> MGSSHHHHHHSQDPANRNVPIPRRQLYIGGEWREPVKKNRIPIINPATEEIIGDIPAATAEDVDIAVEAARKAIARDDWGSTTGAQRAKYLRAIAAKVLEKKSVLATLESLDSGKTLYESAADMDDVAGCFEYYAGLAEALDSRRMTPVNLNSDSYKSYVLREPLGVVGLITPWNYPLLMAIWKVAPALAAGCAAILKPSELASITCLELGEICREIGLPSGALNILTGLGPEAGGPLASHPHVDKISFTGSGPTGSKIMTAAAQLVKPVSLALGGKSPIVVFDDIDNLDIAAEWTLFGIFANTGQVCSATSRLIVQENIASAFMDRLLKWTKNIKISDPL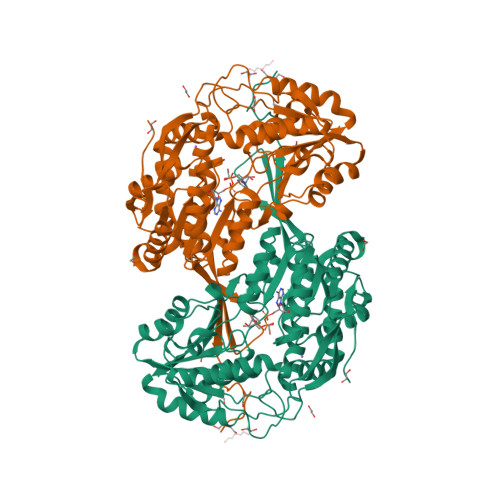EEDCKLGPVVSAGQYEKVLKFISNAKSEGATILCGGERPQHLKKGYYVQPTIITDVNTSMEIWKEEVFGPVLCVKTFKTEEQAIELANDTKYGLGAAVMSKDVKRCERFTKAFQTGIIWINCSQPTFNELPWGGKKRSGFGRDLGKWGLENFLNIKQVTEYTSAEPLAFYKSP In a wide variety of bacterial restriction–modification systems, a regulatory ‘controller’ protein (or C-protein) is required for effective transcription of its own gene and for transcription of the endonuclease gene found on the same operon. We have recently turned our attention to a new class of controller proteins (exemplified by C.Csp231I) that have quite novel features, including a much larger DNA-binding site with an 18 bp (∼60 Å) spacer between the two palindromic DNA-binding sequences and a very different recognition sequence from the canonical GACT/AGTC. The overall structure of the complex consists of a C-protein dimer bound to a DNA duplex. In the complex, each subunit interacts with the DNA by inserting recognition helix 3 (residues 28–40) of the classical helix–turn–helix motif into the major groove of the DNA either side of the central GAAAA motif.

The best diffracting crystals were obtained using 21 bp duplexes corresponding to the core sequences of the OL and OR operator DNA. The C.Csp231I–21-mer DNA duplex complexes crystallized in three crystal forms. For the OL complexes (space groups P61 and C2), the resolutions obtained were 2.30 and 2.75 Å, respectively, while the OR (P61) crystal form diffracted to a resolution of 1.80 Å. The DNA duplex in both complexes is significantly distorted from canonical B-form DNA, with a bend of 39 and 43° for the complexes with OL and OR, respectively, similar to the value (41°) observed in complexes of C.Esp231I with the OL operator. The bend is stabilized by amino-acid contacts to the DNA backbone: principally electrostatic interactions with the phosphate groups on either side of the recognition site. A comparison between the OL and OR structures reveals minor conformational differences, and these are principally in the flexible C-terminal region (residues 86–95); the latter are unlikely to be significant given the flexibility of this region of the protein. There are no base-specific contacts with A9/T13 in OR (or the equivalent G9/C13 in OL), which is the only site within the 15 bp core sequence that differs between the two binding sites. The same is true for the A2/T20 (C2/G20 in OL) and C19/G3 (T19/A3 in OL) base pairs that lie outside the recognition site. This is consistent with the DNA-binding affinity at theses two sites being effectively identical. EMSA analysis of C-protein binding to the left and right operators showed no differences in affinity between the two sites (data not shown).

>[2x]MLIRRLKDARLRAGISQEKLGVLAGIDEASASARMNQYEKGKHAPDFEMANRLAKVLKIPVSYLYTPEDDLAQIILTWNELNEQERKRINFYIRKKAK> MGRQWEEARALGRAVRMLQRLEEQCVDPRLSVSPPSLRDLLPRTAQLLREVAHSRREAGGGGPGGPGGSGDFLLIYLANLEAKSRQVAALL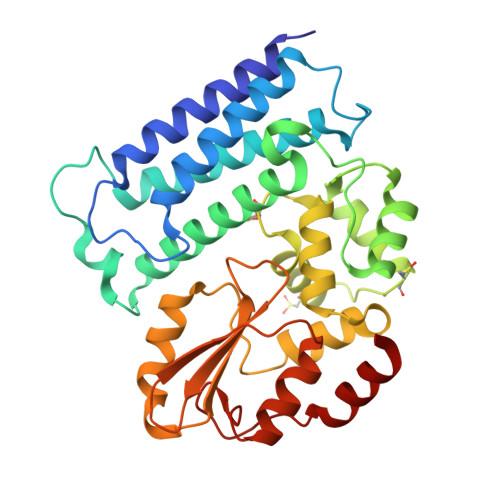PPRGRRSANDELFRAGSRLRRQLAKLAIIFSHMHAELHALFPGGKYCGHMYQLTKAPAHTFWRESCGARCVLPWAEFESLLGTCHPVEPGCTALALRTTIDLTCSGHVSIFEFDVFTRLFQPWPTLLKNWQLLAVNHPGYMAFLTYDEVQERLQACRDKPGSYIFRPSCTRLGQWAIGYVSSDGSILQTIPANKPLSQVLLEGQKDGFYLYPDGKTHNPDLTELGAENLYFQ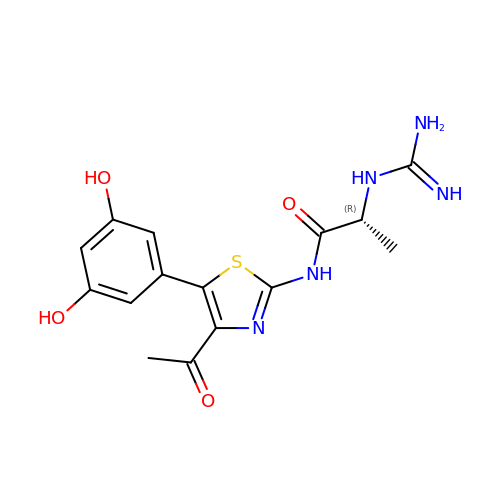(2~{R})-~{N}-[5-[3,5-bis(oxidanyl)phenyl]-4-ethanoyl-1,3-thiazol-2-yl]-2-carbamimidamido-propanamide | C15 H17 N5 O4 S | UGPBIUVAGLINNK-ZCFIWIBFSA-N> MLSKEVVKLLNEQINKEMYAANLYLSMSSWCYENSLDGAG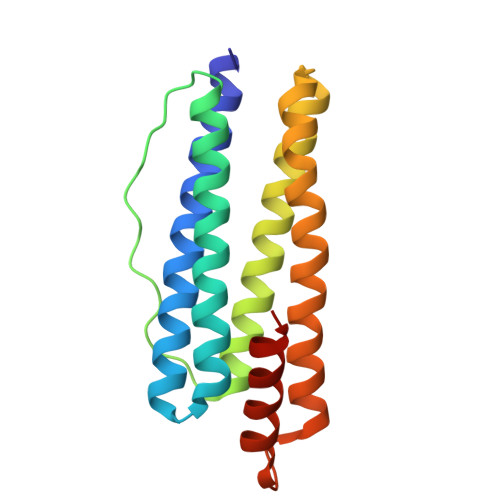AFLFAHASEESDHAKKLITYLNETDSHVELQEVKQPEQNFKSLLDVFEKTYEHEQFITKSINTLVEHMLTHKDYSTFNFLQWYVSEQHEEEALFRGIVDKIKLIGEHGNGLYLADQYIKNIALSRKK>[2x]MMKPEDVIKEQCARAKVVAELWHGFTGGAPKAALENLVVEFNKAQQGRCVRPVPQGGYRDLSTKIKAAFAAGKVPTMAQAFENNIALYLEAKALLPIES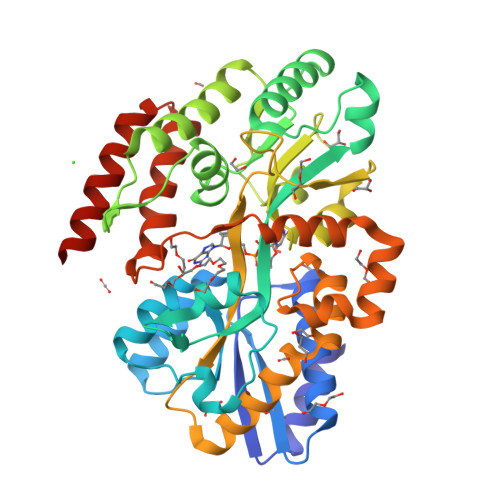LGVKLQGVNLTFLNAVRFGGVVYGVPFNKSIQVLYYNKDLLKKHGVPVPATLEEFVAAAKKLSRAEGGPVYWFQPDASTFAYFFFNLGGSYLKDGKLVLNSKEAVEALTLLQNGVKEGWAKPITSGYINQNLGSGPYAFSVDTSAGYTYYLRAAKFDLGVATLPGRTKGQPGYGLVQGTNLVVFRQASKEEQAVAKDFLEFVLSPRAQAVFATATGYVPVTEGALKDPVYQAYAAENPDYATIVRQSRYAKFEPALAEWEQIRFDILGQAIKEAILNKADPKAALDRAQKLAEDLLSSRTRHHHHHH> ENSLSTTSKSKRQVIVPVCMPKIHYSPLKTGLCYDVRMRYHAKIFT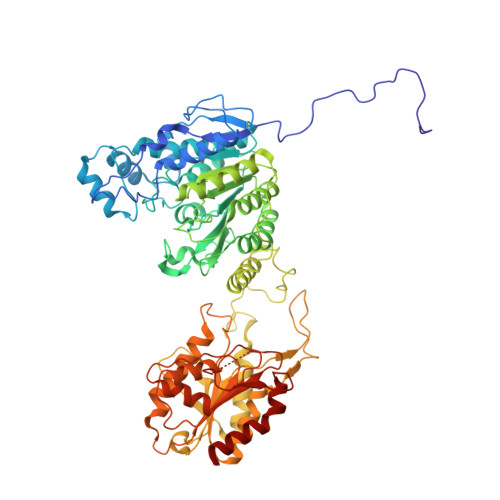SYFEYIDPHPEDPRRIYRIYKILAENGLINDPTLSGVDDLGDLMLKIPVRAATSEEILEVHTKEHLEFIESTEKMSREELLKETEKGDSVYFNNDSYASARLPCGGAIEACKAVVEGRVKNSLAVVRPPGHHAEPQAAGGFCLFSNVAVAAKNILKNYPESVRRIMILDWDIHHGNGTQKSFYQDDQVLYVSLHRFEMGKYYPGTIQGQYDQTGEGKGEGFNCNITWPVGGVGDAEYMWAFEQVVMPMGREFKPDLVIISSGFDAADGDTIGQCHVTPSCYGHMTHMLKSLARGNLCVVLEGGYNLDAIARSALSVAKVLIGEPPDELPDPLSDPKPEVIEMIDKVIRLQSKYWNCFRRRHANSGCNFNEPINDSIISKNFPLQKAIRQQQQHYLSDEFNFVTLPLVSMDLPDNTVLCTPNISESNTIIIVVHDTSDIWAKRNVISGTIDLSSSVIIDNSLDFIKWGLDRKYGIIDVNIPLTLFEPDNYSGMITSQEVLIYLWDNYIKYFPSVAKIAFIGIGDSYSGIVHLLGHRDTRAVTKTVINFLGDKQLKPLVPLVDETLSEWYFKNSLIFSNNSHQCWKENESRKPRKKFGRVLRCDTDGLNNIIEERFEEATDFILDSFE> S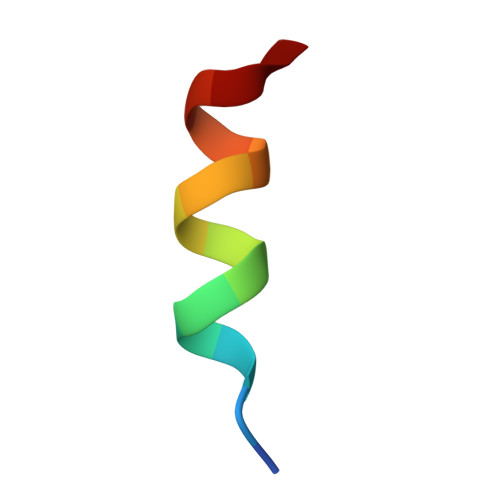SSPGQLLDILNSK> MKRILVVDDEPNIRELLKEELQEEGYEIDTAENGEEALKKFFSGNYDLVILDIEMPGISGLEVAGEIRKKKKDAKIILLTAYSHYRSDMS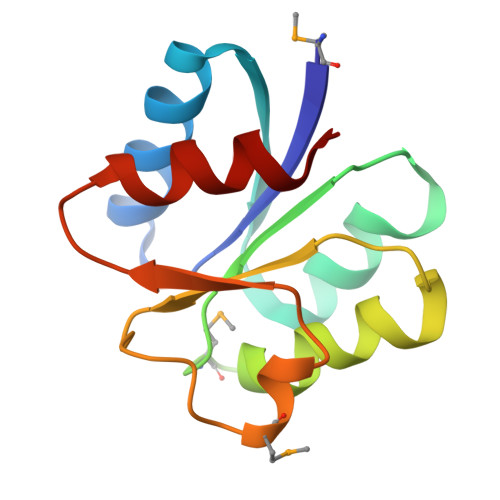SWAADEYVVKSFNFDELKEKVKKLLS>[2x]MHHHHHHLKFMLDTNICIFTIKNKPASVRERFNLNQGKMCISSVTLMELIYGAEKSQMPERNLAVIEGFVSRIDVLDYDAAAATHTGQIRAELARQGRPVGPFNQMIAGHARSRGLIIV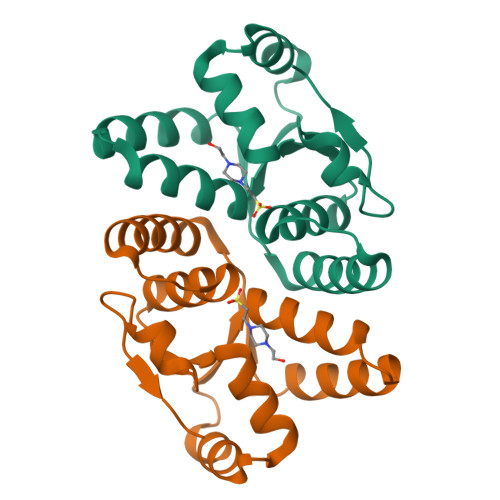TNNTREFERVGGLRTEDWS>[2x]ETGCNKALCASDVSKCLIQELCQCRPGEGNCSCCKECMLCLGALWDECCDCVGMCNPRNYSDTPPTSKSTVEELHEPIPSLFRALTEGDTQLNWNIVSFPVAEELSHHENLVSFL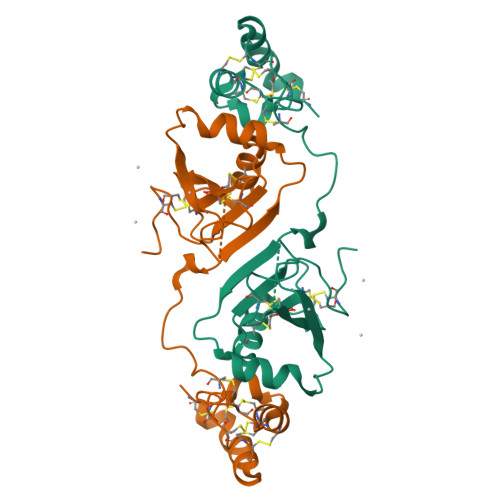ETVNQPHHQNVSVPSNNVHAPYSSDKEHMCTVVYFDDCMSIHQCKISCESMGASKYRWFHNACCECIGPECIDYGSKTVKCMNCMFGTKHHHHHH The wall teichoic acid (WTA) is a major cell wall component of Gram-positive bacteria, such as methicillin-resistant Staphylococcus aureus (MRSA), a common cause of fatal clinical infections in humans. Thus, the indispensable ABC transporter TarGH, which flips WTA from cytoplasm to extracellular space, becomes a promising target of anti-MRSA drugs. In S. aureus, ABC transporter TarGH is indispensable for the transmembrane flipping of WTA precursor, an N-acetylglucosamine (GlcNAc)-modified ribitol-phosphate (RboP) polymer covalently linked to the UND-PP moiety, out of the cell membrane.

Using the cryo-electron microscopy (cryo-EM) technique, we solved the structure of A. herbarius TarGH at an overall resolution of 3.9 Å, with the catalytic residue Glu169 mutated to Gln. In the absence of ATP, TarGH adopts an inward-open conformation. The distance between the hydroxyl groups of Ser64 on Walker A from one NBD and Ser146 on the signature motif from the other is about 6 Å, suggesting a resting state of TarGH ready for ATP binding. Similar to other type II ABC exporters, the TMDs of TarGH consist of 6 + 6 transmembrane helices (TMs) without domain swapping. Using the program Caver 3.0.1 (25), with the probe radius set to 1.1 Å, we simulated two back-to-back L-shaped substrate tunnels, each of which has a horizontal entrance along the membrane-cytosol interface and a vertical path through the cell membrane. The turn is surrounded by a line of positively charged residues, Lys93, Arg98, Arg100, Lys120, Arg175, and Arg186, whereas the transmembrane path is mainly composed of hydrophobic residues, such as Tyr51, Phe55, Trp81, Phe82, Val84, Leu89, Leu189, Tyr190, and Trp196. Scanning along the vertical path, we found a constrained bottleneck at the tunnel exit toward the extracellular space, which is guarded by Tyr51, Phe55, and Tyr190 from each TMD. Remarkably, four of these residues, Phe55, Trp73, Phe82, and Tyr190, on each TMD form a hydrophobic pocket, which is occupied by the loop between TM5 and EH1 that harbors another Targocil-resistant residue, Leu195. The ATP-free TarGH adopts a resting state, with the substrate tunnel closed at the exit and open at the entrance (state 1), as shown in our cryo-EM structure. At this state, the latch loop blocks the exit and functions as an autoinhibitor that mimics the exogenous inhibitor Targocil, while the entrance formed by the GL and LoopTM4-TM5 is open and ready for substrate recognition and binding.

>[2x]MEHAVIVENVTKKYKLFKRTSERLLDMILPGGYGEDFYALRNVSFTADKGDVIGIVGVNGSGKSTLSNIIAGILPPTSGTIKIDGQASLIAISSGLNNQLTGRENIELKCLMLGFSKKQIRAMEPDIIEFADIGKFIDQPVKTYSSGMKSRLGFAISVNIDPDVLVIDEALSVGDQTFADKCLDKMNEFKERGKTIFFISHSIGQVKSFCEKALWLEYGEVRGYGTVAEIIPQYEKFLKEYRAMSDKEKRQYKERVMRKQQGEFLQAAVK;>MGHHHHHHHHHHMRSAVTVLMEHIRNLYLIRRLSLFELKSDNSNQYLGILWEIINPMIQIAIYWFVFGYGIRGRHPVGHIPFILWMLAGMTVWFFVNQAVLQASKSVYTRIRMVAQMNFPISVIPTYVITAKFYQHLMLLAVIFIIFQFTPYHVSVYLVQLPYYMFGLLALLVSFSLITSTLATVVRDVQMIVQSLVRILLYLTPLLWDPSHLPHLVQVIMRLNPLYYIVEGYRSALLGTSWYLVDHASYTVYFWVVVILFFVFGSMVHLKFRAHFVDYM[2x]(3~{S},4~{R})-oxolane-3,4-diol | C4 H8 O3 | 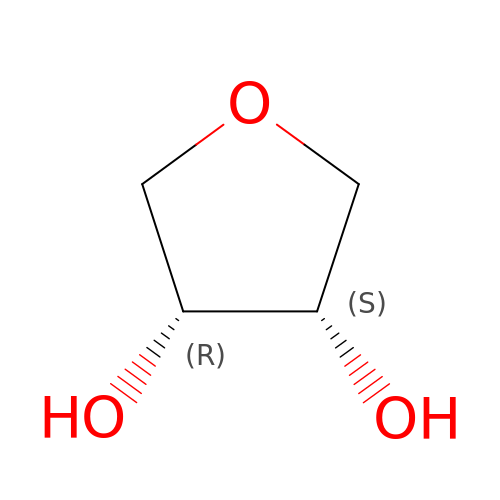SSYDTHANSGMJTP-ZXZARUISSA-N>PADQTNRTSHPLPQGVNRYFVVKSNNRENFELSVQQGVWATQRSNEAKLNEAFDSVENVILIFSVNRTRHFQGCAKMTSRIGGYIGGGNWKHEHGTAQYGRNFSVKWLKLCELSFHKTRNLRNPYNENLPVKISRDCQELEPSVGEQLASLLYLEPD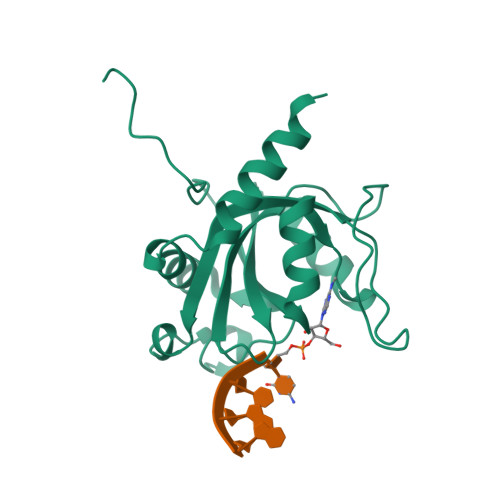SELMAISIAAEAKREEEKAKGVN[4x]> XPPGP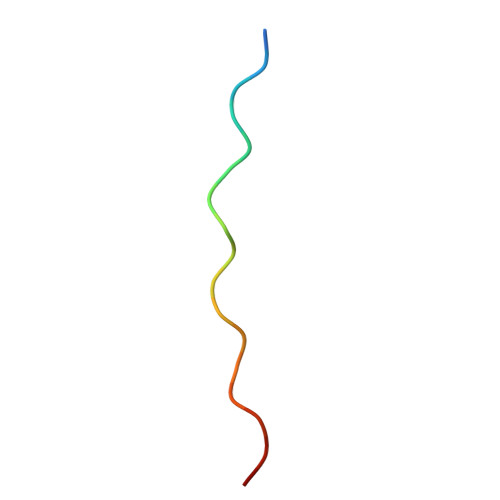PGPTGPRGPPGPPX>[2x]MPQDVDFHIPLPGRQSPDHARAEAEQLAWPRSLGLIRSDAAAERHLRGGYADLASRFYPHATGADLDLGVDLMSWHFLFDDLFDGPRGENPEDTKQLTDQVAAALDGPLPDTAPPIAHGFADIWRRTCEGMTPAWCARSARHWRNYFDGYVDEAESRFWNAPCDSAAQYLAMRRHTIGVQPTVDLAERAGRFEVPHRVFDSAVMSAMLQIAVDVNLLLNDIASLEKEEARGE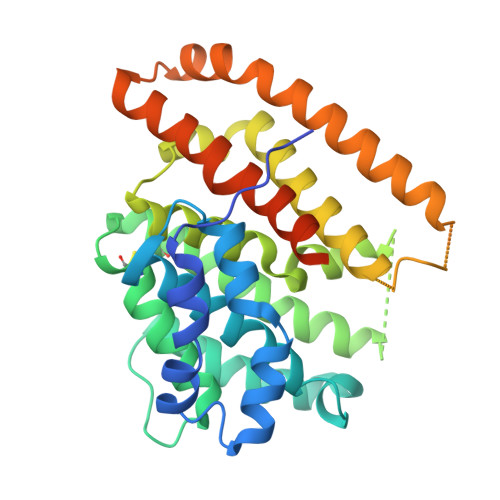QNNMVMILRREHGWSKSRSVSHMQNEVRARLEQYLLLESCLPKVGEIYQLDTAEREALERYRTDAVRTVIRGSYDWHRSSGRYDAEFALAAGAQGYLEELGSSAH> MASMTGGQQMGRGSDPNTSKQSNDYKYDINTSCISREGTTTLERKNLILCHSGKLEDKYIIDEKLGQGTYGCVYKGIDKVTNQLYAIKEEKKDRLKNINRFFQEIEIMKKLDHPNIVKLYETYENDNYIYLIMELCSGRELFDSIIENGSFTEKNAATIMKQIFSAIFYLHSLNIVHRDLKPENFLFQSENKDSLLKIIDFGLSKNLGTGEFTTTKAGTPYYVAPQVLDGKYDKKCDIWSSGVIMYTLLCGYPPFYGDTDNEVLKKVKKGEFCFYEND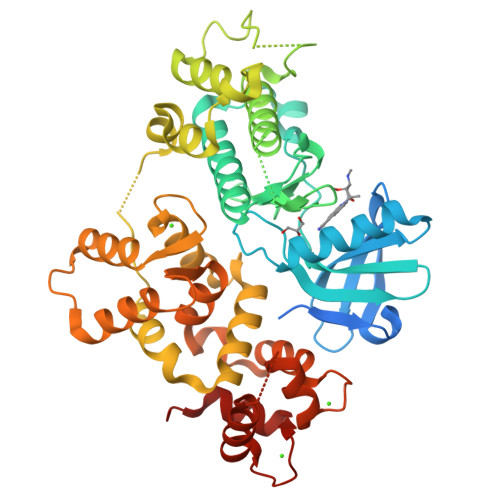WGSISSDAKNLITKLLTYNPNERCTIEEALNHPWITQMTKSHEHVELSSTLLKNLKNFKKENELKKIALTIIAKHLCDVEINNLRNIFIALDVDNSGTLSSQEILDGLKKIGYQKIPPDIHQVLRDIDSNASGQIHYTDFLAATIDKQTYLKKEVCLIPFKFFDIDGNGKISVEELKRIFGRDDIENPLIDKAIDSLLQEVDLNGDGEIDFHEFMLMMSKLEHHHHHH>[4x]ADTIVAVELDTYPNTDIGDPNYPHIGIDIKSVRSKKTAKWNMQNGKVGTAHIIYNSVGKRLSAVVSYPNGDSATVSYDVDLDNVLPEWVRVGLSASTGLYKETNTILSWSFTSKLKSNSTHETNALHFMFNQFSKDQKDLILQGDATTGTDGNLELTRVSSNGSPQGSSVGRALFYAPVHIWESSAVVASFDATFTFLIKSPDSHPADGIAFFISNIDSSIPSGSTGRLLGLFPDAN

We report here the crystal structure of a native and complexed lectin isolated from Canavalia gladiata seeds, describing a new binding pocket in ConA-like lectins, which may be related to pathogen resistance, a site where a non-protein amino acid, such as α-amino butyric acid, can bind. The most recent accepted definition establishes lectins as proteins with at least one non-catalytic domain able to recognize and bind reversibly to specific mono and oligosaccharides. The oligomeric structures of CGL and CGL-αMM involve two 'canonical' dimers, and these dimers are associated by salt bridges between β-strands. In both CGL crystal structures, the amino acids involved in metal binding are conserved.

The crystal structure of native CGL and in complex with α-methyl-mannoside (CGL-αMM) provides a new source of information for the understanding of lectins and reveals a new binding site for a non protein amino acid at the monomers contact interface of each canonical dimer of leguminous lectins. The overall structure of native CGL and CGL-αMM has been refined at the 2.3 Å and 2.31 Å resolutions, respectively. Commonly, five to eight H-bonds occur between monosaccharides and the Diocleinae lectin domain amino acids Asn14, Leu99, Tyr100, Asp208 and Arg228; CGL-αMM displays an alpha-methyl-mannoside recognition involving seven H-bonds with specific amino acid residues and another with a water molecule. The nitrogen side chain of Asn14 forms a single H-bond with αMM O4 oxygen at 2.6 Å; the main chain nitrogens of Leu99 and Tyr100 are connected with αMM O5 and O6 oxygens. Oxygens from Asp 208 side chain are the CGL closest atoms from the αMM. They are positioned at 2.5 Å from O7 and 2.7 Å from O6, and the main chain nitrogen of Arg 228 makes a 2.9 Å H-bond with αMM O3 oxygen. Abu was found at the monomers contact interface of CGL-αMM. Abu ligand is accessible to the solvent surface by the carboxyl group and interacts with one chain through hydrogen bond with Asp139 and an interstitial water molecule, which interacts with Asn 124 and with the other chain through hydrogen bonds with Ala 125 and with another interstitial water interacting with Gln 137, and through hydrophobic interaction with Leu126 and Val 179. The presence of Abu at the monomers interface increased the intermolecular contacts and strongly stabilized the canonical dimers. In addition, residues corresponding to Leu 126 and Val 179, which are effective in hydrophobic anchoring of Abu, and the ones corresponding to Asp 139 and Gln 137, responsible by hydrophilic contacts, are highly conserved in spite of the relative phylogenetic distance of these leguminous tribes.N-OMEGA-NITRO-L-ARGININE 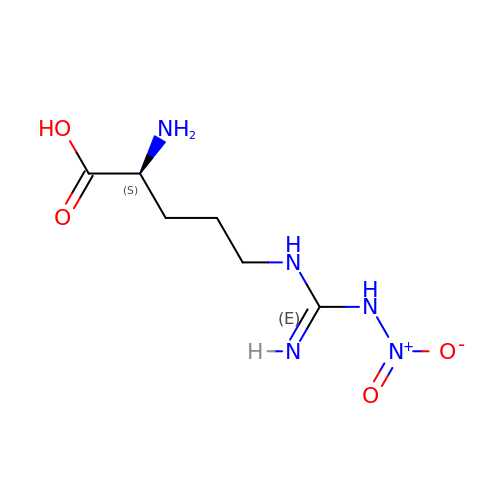| C6 H13 N5 O4 | MRAUNPAHJZDYCK-BYPYZUCNSA-N>[2x]SNAMLAF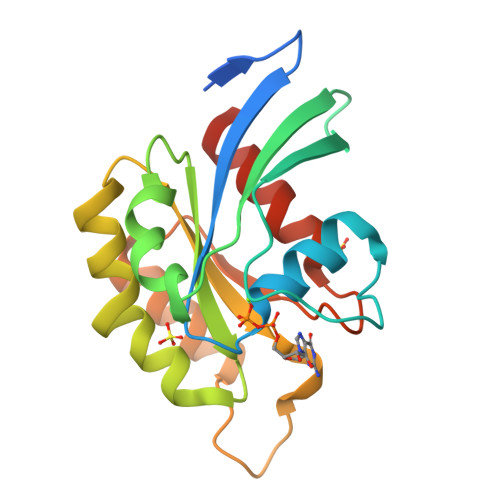SDMNTGAGKIENGKKALKIVVVGDGAVGKTCLLLAFSKGEIPTAYVPTVFENFSHVMKYKNEEFILHLWDTAGQEEYDRLRPLSYADSDVVLLCFAVNNRTSFDNISTKWEPEIKHYIDTAKTVLVGLKVDLRKDGSDDVTKQEGDDLCQKLGCVAYIEASSVAKIGLNEVFEKSVDCIFSNKPVPK>[2x]PETETEVTPIQQ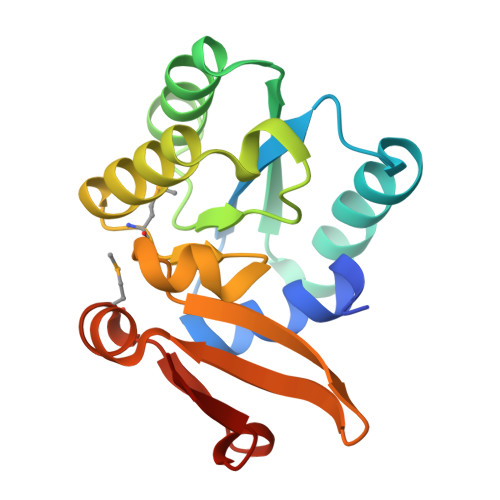LFLIKELKPGIARIGVIWDKNAANRDEVLPQLQRASAATGIKVVVAEVASLQEVAPQFRTLLRDHQVEALWVLEESGLLGQAAARSFLIKNATQAGMPVFAPSETWLKEGACVTWRKDAEGIRLVVNKAVAEAMGITIPAKYQDRTAFLAMN N-(1-{2-[(cyclopropanesulfonyl)amino]-1,3-thiazol-4-yl}cyclopropyl)-5-(6-ethoxypyrazin-2-yl)pyridine-2-carboxamide | C21 H22 N6 O4 S2 | 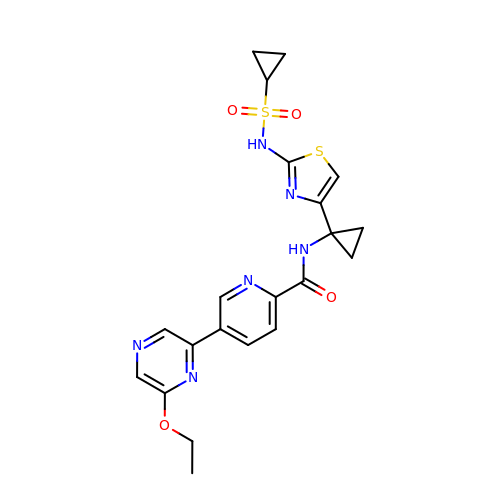VIXAYXSBOOBUNP-UHFFFAOYSA-N>[2x]GGGNEEFRPEMLQGKKVIVTGASKGIGREMAYHLAKMGAHVVVTARSKETLQKVVSHCLELGAASAHYIAGTMEDMTFAEQFVAQAGKLMGGLDMLILNHITNTSLNLFHDDIHHVRKSMEVNFLSYVVLTVAALPMLKQSNGSIVVVSSLAGKVAYPLVAAYSASKFALDGFFSSIRKEYSVSRVNVSITLCVLGLIDTETAMKAVSGIVHMQAAPKEECALEIIKGGALRQEEVYYDSSRWTTLLIRN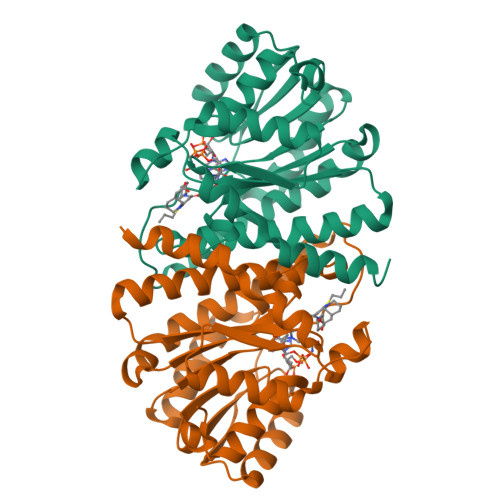PSRKILEELYSTSYNWDRFINK>[2x]MIELRNLTKWYPTPHGRRYVFRNLNFRFPDDVSIGLIGRNGAGKSTLMRLLGGIEAPNEGEVVTDVSISWPVGLSGGFQGSLTARENVKFVCRIYGTSHEDMLRKVRFVEEFAEIGEHFDLPMKTYSSGMRSRVAFGLSMAFDFDYYLIDEAMAVGDAQFRAKSRAVFDSRVGQANMILVSHNMNDIKEY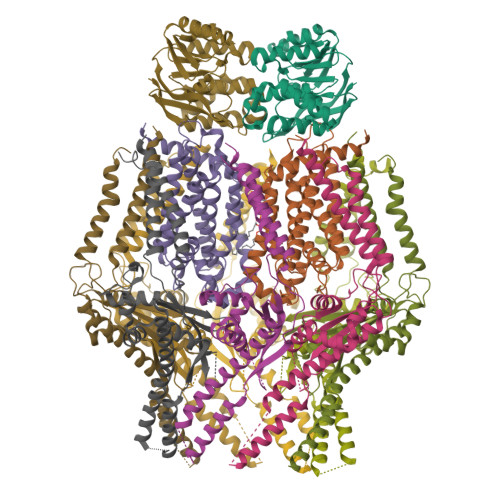CDVVVLVDQGQATLYEDVEAGIAAYQGSLKKAAAKPDYKDDDDK;>MGKIHLAVSERSPRVKRSPWQIQQAVLFALFLRELKTRLGGRWLGVFWVLLEPVAHIAVMTTLFSLAHRAAMPSIEYPVFLITGLIPFFMFRGLVTRLMEAIDSNRGLFAYRQVKPIDTVIARAMLEISLQSIVYLIALGTLGWLGFHFLPVRALELAGVSAVLIMLGASLGLFFAVVTNEIPQARAIVRISLLPLYFVSGVIFPVHTIPPQYLPLLQLNPVLHLIELSRASFFPQYRVLQGINLAYPAGFALLSLFLALMLYRLRRHQLASVV[2x];>[8x]MGKIHMKLVSRLTAKRLQWALVYLPMLVATVYFLVFSADRYVSESVITVRQTSSNAPTGGMSGAALLLAGLTPASREDTCYLQTYIHSMGLLQKLDQQLKLREHFGTPLRDPLFRLWGGTSQEWFLEYYRSRVEVLMDDICGLLTVRVQGFEPEFAQALNRAILEESERFVNELSHRMAREQGQFAEAELERATARLQEAKRQLIAFQAKHKLLDPLAQAQATGTLTAELQAALTRQEAELRNALTYLNEDSYQVKALRSQINALRQQIDEERLRATAGKNGDRINAVAAEFHDLQLQVGFAEDAYKLALAAVESARIEATRKLKSLVVVEPPVLPEIAEYPRRWYNLATLLVVCCLIYGVVSLVVATIRDHQDGSGSGSHHHHHHHHHH> QGHLRSGPRIFAVWKGHVGQDRVDFGQTEPHTVLFHEPGSSSVWVGGRGKVYLFDFPEGKNASVRTVNIGSTKGSCLDKRDCENYITLLERRSEGLLACGTNARHPSCWNLVNGTVVPLGEMRGYAPFSPDENSLVLFEGDEVYSTIRKQEYNGKIPRFRRIRGESELYTSDTVMQNPQFIKATIVHQDQAYDDKIYYFFREDNPDKNPEAPLNVSRVAQLCRGDQGGESSLSVSKWNTFLKAMLVCSDAATNKNFNRLQDVFLLPDPSGQWRDTRVYGVFSNPWNYSAVCVYSLGDIDKVFRTSSLKGYHSSLPNPRPGKCLPDQQPIPTETFQVADRHPEVAQRVEPMGPLKTPLFHSKYHYQKVAVHRMQASHGETFHVLYLTTDRGTIHKVVEPGEQEHSFAFNIMEIQPFRRAAAIQTMSLDAERRKLYVSSQWEVSQVPLDLCEVYGGGCHGCLMSRDPYCGWDQGRCISIYSSERSVLQSINPAEPHKECPNPKPDKAPLQKVSLAPNSRYYLSCPMESRHATYSWRHKENVEQSCEPGHQSPNCILFIENLTAQQYGHYFCEAQE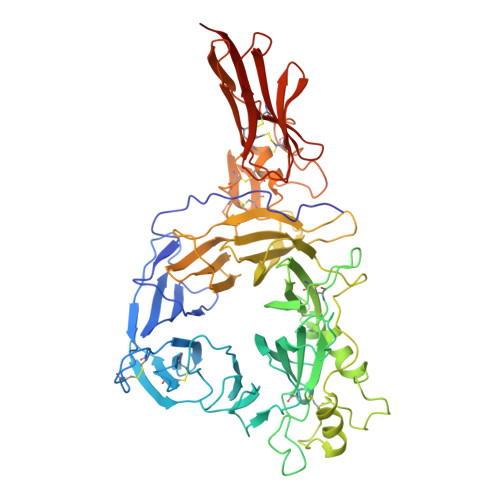GSYFREAQHWQLLPEDG> MIGVNRMTEASTYIGTVQDVNGANIRVVLDINTISSLKFVDGQGYRIGQIGSFVRIPIGYINLFGIVSQVGAGAVPDKLLEVEPYGHRWISVQLVGEEGIKKEFERGVSQYPTIGDKVHIVTEPDLKKIYGTQNKKYISLGNIASVDSIPALVNIDTLVTRHSAVLGSTGSGKSTTVTSILQRISDMSQFPSARIIVFDIHGEYAAAFKGKAKVYKVTPSNNELKLSIPYWALTCDEFLSVAFGGLEGSGRNALIDKIYELKLQTLKRQEYEGINEDSLTVDTPIPFSIHKLWFDLYRAEISTHYVQGSHSEENEALLLGEDGNPVQKGDSLKVVPPIYMPHTQAQGATKIYLSNRGKNIRKPLEGLASLLKDPRYEFLFNADDWSVNLDGKTNKDLDALLETWVGS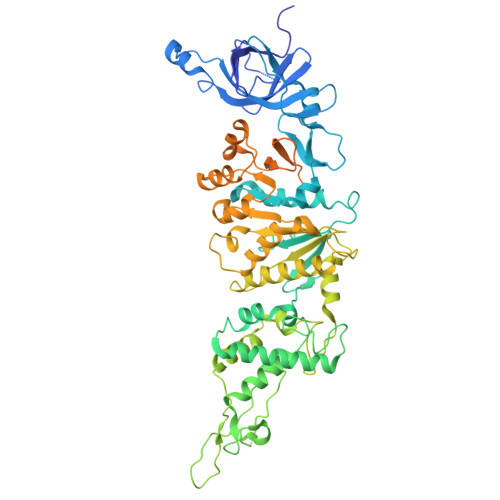EESISIFDLSGMPSSILDTLIGILIRILYDSLFWSRNQPEGGRERPLLVVLEEAHTYLGKDSRGIAIDGVRKIVKEGRKYGIGMMLVSQRPSEIDSTILSQCGTLFALRMNNSSDRNHVLGAVSDSFEGLMGMLPTLRTGEAIIIGESVRLPMRTIISPPPFGRRPDSLDPDVTAKWSNNRVQGDYKEVLTLWRQKKVRSQRIVENIKRLPVVNEGEMTDMVREMVTSSNILSIGYEADSMTLEIEFNHGLVYQYYDVPETLHTELLAAESHGKFFNSQIKNNYRFSRI>[2x]MRAVNWNKKEDDFSLMFWKQNIAQFWTEEEIAVSSDKNTWVQLSKEEQIAYKRVLGGLTLLDTKQGGEGMPLVLVHLENLQAKSVLAFMGAMEEVHAKSYSHIFTTLATEEEIDEIFDWVDTHPLLEKKAGIITSYYRRLLKPEVTKKELYMAMVASVFLESYLFYSGFFYPLYLAGQGKLTASGEIINLIIRDESIHGVFVGILAQQIF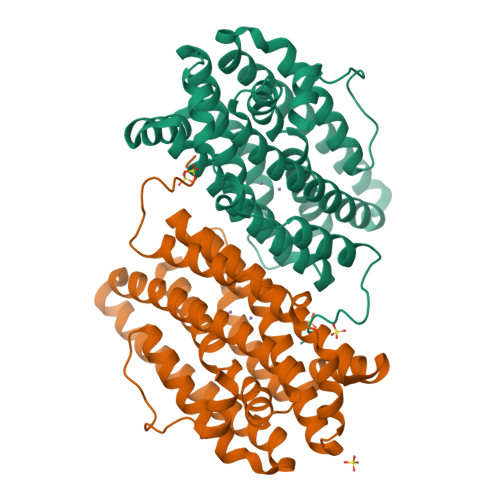AELSAEDQQEVQKETQELLMELYEIEMAYTEEIYTSIGLVEDVNRFVRYNANKGLMNLGLEPKFEEEEINPIVLNGLRTDTKNHDFFSVKGNGYVKATNVEKLSDDDFVFNF>[3x]GLAEKLVPAKKVKNGVLYKSGHIKVSNV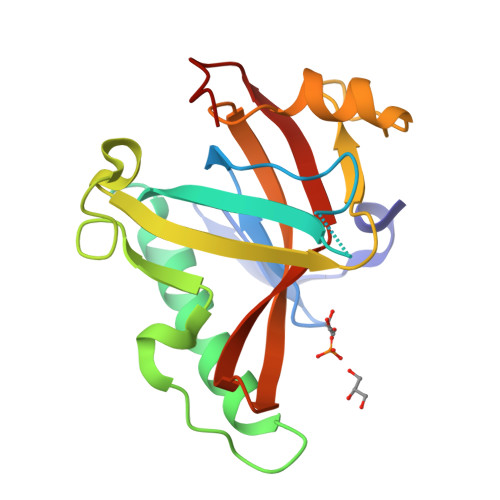RCSYPHLDKPYGGEDGGEPKYSITLLMPKDTHGAIKKIIDEQIELTKKNHKTGALKVAPSMLFIKDGDVDFPDKPECEGMWVISARESTRPDVLNMEREELESPNEIAEEIYGGCWVSSVIRPWSQENKYGKRINANLLSVLKRKDDEPFGE(2S,3R)-4-(2-amino-2-oxoethoxy)-3-(dihydroxy-lambda~4~-sulfanyl)-3-methyl-4-oxo-2-{[(1E)-3-oxoprop-1-en-1-yl]amino}butanoic 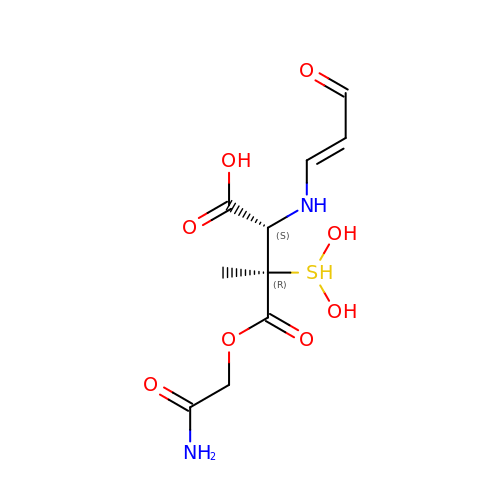acid | C10 H16 N2 O8 S | MGCULWRADYDHMU-SSWUGZLXSA-N AChBPs are homopentameric, water-soluble homologs of the ligand-binding domain of LGICs and well-established structural surrogates for nicotinic acetylcholine receptors (nAChR). Importantly, AChBPs can bind nAChR-specific ligands and induce similar conformational changes as in the membrane bound receptors. LGICs are activated by ligands binding at subunit interfaces of their extracellular domains, thereby inducing conformational changes that affect the structure of a central pore and its ability to transport ions through the membrane. Additional density was found in all structures at the interface between the subunits in the orthosteric agonist and antagonist binding site, next to loop C in which the respective ligands could be modelled.

In total, five structures of Ls-AChBP in complex with a ligand were successfully solved. The electron density in the binding site region was generally poor, indicating that compounds may have had several binding modes in the site. A computational alignment and superimposition of AChBP taken from the protein–ligand complexes and the apo structure showed that there were no large global conformational changes in any of the structures upon ligand binding. However, there were small changes in the loop C region of the crystal structures of Ls-AChBP. When comparing the protomers in complex with a ligand we observed that loop C moves differently upon binding of different compounds. Notably, binding of FL1888, VUF24234 and VUF6105 results in a movement of the loop closer to the compound, while binding of FL1856, FL3044, FL1613 and FL1909 does not have the same effect. The plot indicates that binding of nicotine, FL1613, FL1909, FL1856 and FL3044 do not result in any significant conformational changes in this region, while binding of FL1888, VUF24234 and VUF6105 do.

>[20x]MRRNIFCLACLWIVQACLSLDRADILYNIRQTSRPDVIPTQRDRPVAVSVSLKFINILEVNEITNEVDVVFWQQTTWSDRTLAWNSSHSPDQVSVPISSLWVPDLAAYNAISKPEVLTPQLARVVSDGEVLYMPSIRQRFSCDVSGVDTESGATCRIKIGSWTHHSREISVDPTTENSDDSEYFSQYSRFEILDVTQKKNSVTYSCCPEAYEDVEVSLNFRKKGRSEILGSHHHHHH> VFHKIRNEDLIFNESLGQGTFTKIFKGVRREVGDYGQLHETEVLLKVLDKAHRNYSESFFEAASMMSKLSHKHLVLNYGVCVCGDENILVQEFVKFGSLDTYLKKNKNCINILWKLEVAKQLAAAMHFLEENTLIHGNVCAKNILLIREEDRKTGNPPFIKLSDPGISITVLPKDILQERIPWVPPECIENPKNLNLATDKWSFGTTLWEICSGGDKPL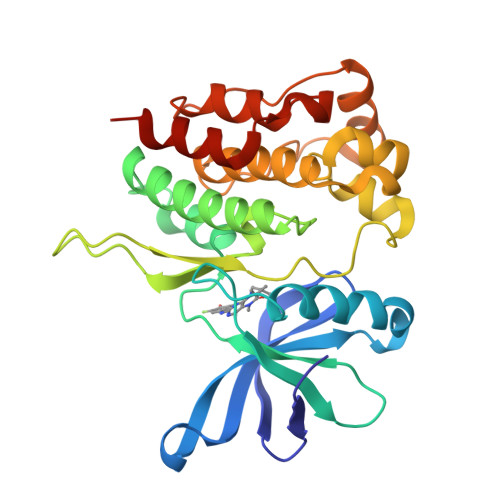SALDSQRKLQFYEDRHQLPAPKAAELANLINNCMDYEPDHRPSFRAIIRDLNSLFTPD>[2x]MLTEGISIQSYDGHTFGALVGSPAKAPAPVIVIAQEIFGVNAFMRETVSWLVDQGYAAVCPDLYARQAPGTALDPQD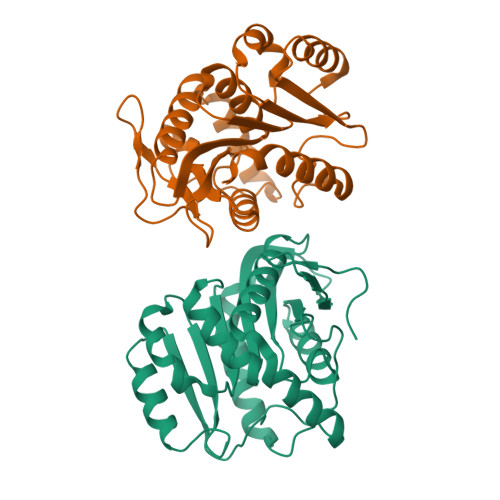ERQREQAYKLWQAFDMEAGVGDLEAAIRYARHQPYSNGKVGLVGYSLGGALAFLVAAKGYVDRAVGYYGVGLEKQLNKVPEVKHPALFHMGGQDHFVPAPSRQLITEGFGANPLLQVHWYEEAGHSFARTSSSGYVASAAALANERTLDFLAPLQSKKP>HTSPLLAPVRQIHAFGDSYSDNGESQRLTREMLAKGIAGAQALPGEVYWQGRWSNGPTAVEVLARQLGAQLADHAVGGAKSGADNYYGWMSAYRHTGLAGQVDAYLATLDGKPVDGQALHFIFVSANDFFEHEDFAGEQPLEQLAG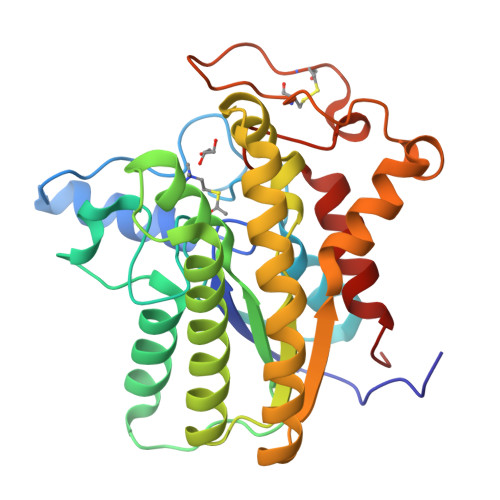SSVANIRAAVQRLGEAGARRFLVVSSTDLSVVPAVVAGNRVERAQRYLQAVNASLPIQLAALRKTRGLELSWFDHLTFSRHLRRNPARYGLVELDAPCQPTQPSVRPACANPDQYYFWDEWNPTRRVHQLAGEAMAARYAR[2x]>LYF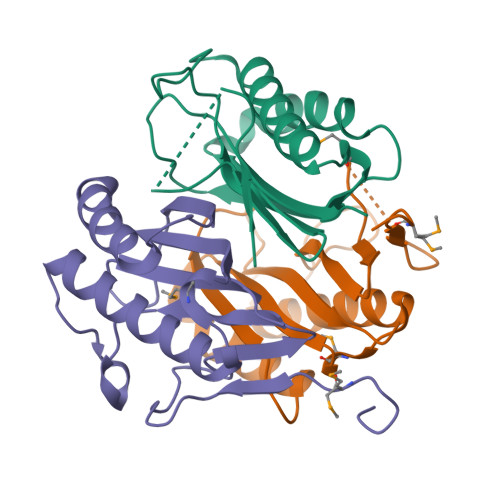QGHMPKSVIIPAGSSAPLAPFVPGTLADGVVYVSGTLAFDQHNNVLFADDPKAQTRHVLETIRKVIETAGGTMADVTFNSIFITDWKNYAAINEIYAEFFPGDKPARFCIQCGLVKPDALVEIATIAHIAK[6x]> MSDGTSQPDSGNAVHSAARVERAADGPGGSGGGGSGGGGVGVSTGSYDNQTHYRALGDGWVE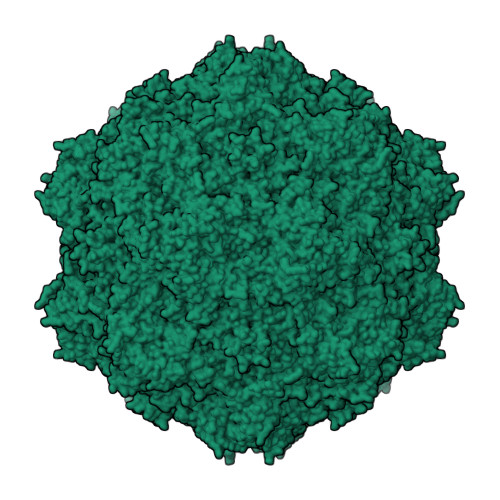ITALATRLVHLNMPKSENYCRIRVHNTTDTSVKGNMAKDDAHEQIWTPWSLVDANAWGVWLQPSDWQYICNTMSQLNLVSLDQEIFNVVLKTVTEQDLGGQAIKIYNNDLTACMMVAVDSNNILPYTPAANSMETLGFYPWKPTIASPYRYYFCVDRDLSVTYENQEGTVEHNVMGTPKGMNSQFFTIENTQQITLLRTGDEFATGTYYFDTNPVKLTHTWQTNRQLGQPPLLSTFPEADTDAGTLTAQGSRHGTTQMGVNWVSEAIRTRPAQVGFCQPHNDFEASRAGPFAAPKVPADITQGVDKEANGSVRYSYGKQHGENWASHGPAPERYTWDETSFGSGRDTKDGFIQSAPLVVPPPLNGILTNANPIGTKNDIHFSNVFNSYGPLTAFSHPSPVYPQGQIWDKELDLEHKPRLHITAPFVCKNNAPGQMLVRLGPNLTDQYDPNGATLSRIVTYGTFFWKGKLTMRAKLRANTTWNPVYQVSAEDNGNSYMSVTKWLPTATGNMQSVPLITRPVARNTY(4S)-4-(decanoylamino)-5-hydroxy-3,4-dihydro-2H-thiophenium | C14 H25 N O2 S | 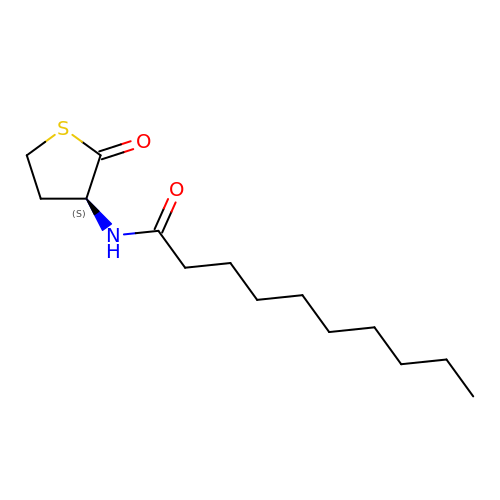PZUMIWRJDZWNPN-LBPRGKRZSA-N>[2x]ACPGIVPRSVWGARETHCPRMTLPAKYGIIIHTAGRTCNISDECRLLVRDIQSFYIDRLKSCDIGYNFLVGQDGAIYEGVGWNVQGSSTPGYDDIALGITFMG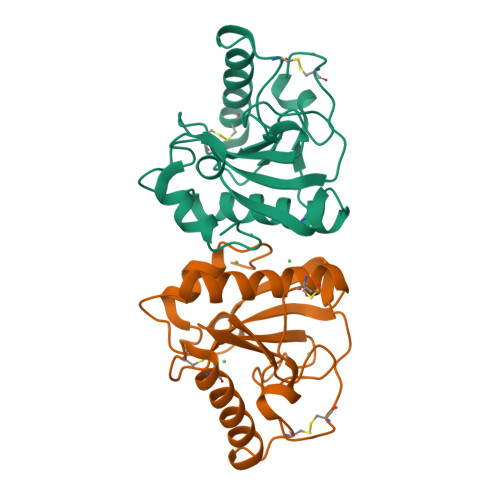TFTGIPPNAAALEAAQDLIQCAMVKGYLTPNYLLVGHSDVARTLSPGQALYNIISTWPHFKH>[4x]ILGGQEAAAHARPYMASVQVNGTHVCGGTLLDEQWVLSAAHCMDGVTDDDSVQVLLGAHSLSAPEPYKRWYDVQSVVPHPGSRPDSLEDDLILFKLSQ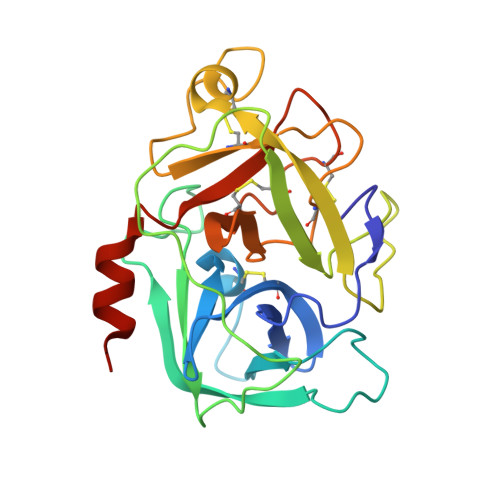NASLGPHVRPLPLQYEDKEVEPGTLCDVAGWGVVTHAGRRPDVLHQLRVSIMNRTTCNLRTYHDGVVTINMMCAESNRRDTCRGDSGSPLVCGDAVEGVVTWGSRVCGNGKKPGVYTRVSSYRMWIENITNGNMTS> GPLGSPQMAQGTLIRVTPEQPTHAVCVLGTLTQLDICSSAPEDCTSFSINASPGVVVDIAHSPPAKKKSTGSSTWPLDPGVEVTLTMKAASGSTGDQKVQISYYGPKTPPVKALLYLTAVEISLCADITRTGKVKPTRAVKDQRTWTWGPCGQGAILLVNCDRDNLESSAMDCEDDEVLDSEDLQDMSLMTLSTKTPKDFFTNHTLVLHVARSEMDKVRVFQATRGKLSSKCSVVLGPKWPSHYLMVPGGKHNMDFYVEALAFPDTDFPGLITLTISLLDTSNLELPEAVVFQDSVVFRVAPWIMTPNTQPPQEVYACSIFENEDFLKSVTTLAMKAKCKLTICPEEENMDDQWMQDEMEIGYIQAPHKTLPVVFDSPRNRGLKEFPIKRVMGPDFGYVTRGPQTGGISGLDSFGNLEVSPPVTVRGKEYPLGRILFGDSCYPSNDSRQMHQALQDFLSAQQVQAPVKLYSDWLSVGHVDEFLSFVPAPDRKGFRLL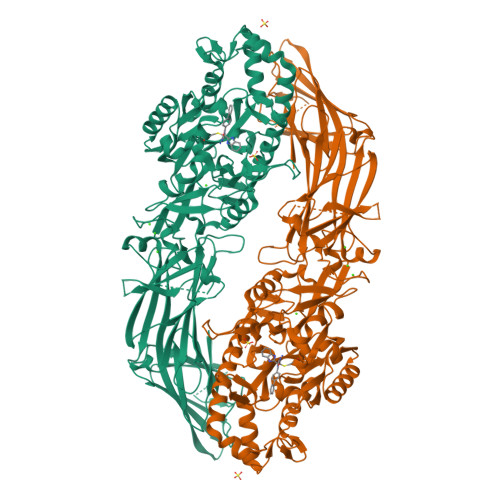LASPRSCYKLFQEQQNEGHGEALLFEGIKKKKQQKIKNILSNKTLREHNSFVERCIDWNRELLKRELGLAESDIIDIPQLFKLKEFSKAEAFFPNMVNMLVLGKHLGIPKPFGPVINGRCCLEEKVCSLLEPLGLQCTFINDFFTYHIRHGEVHCGTNVRRKPFSFKWWNMVP> GKGGKGLGKG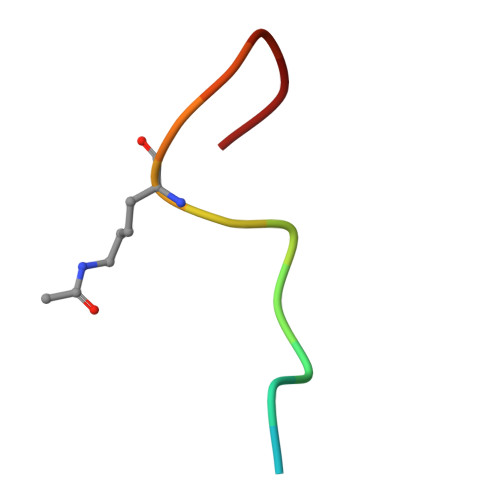GAKR>MAIELWTTRNDTTSVQAFYAAEAGLQKYKAALFQQYVWREQRGGTGGGGGCFTSLARGLDLDRDGTITPFVNNRLVLAQNEVVTDANGNPVGRYTATLYKDAQDDQLFTLVSEGTSGGAKARVQATFRISNSDYLEQAIFAGAGQANKWLNGGATIRGGVYVVGNPNDPDQYVIEANGNFALYNRYDLTTYSEVTNRVEPSYRQVQDLCASLRVQYGKISVGGSTQIGEPNNKVKGVFVGRGAQDITGENVGVCRNNKGVCTEAMGGFDLSDPPPFPTLDAKLDSDACSAYPTWRACLQGKAALRIQRIGNILSVASPPNATLSPSCLQAMQSGTLTLDTQSVDCTFTRLDGSRGGFRYTYTGGQELLEVFGDVVLEGIDAVLNRPVDYRAQSGSAKSATLAVLKLGGNGGNLDINGNLLPDATFGLFPNHALGFVAEGDIYQRGQHVMAPVYAGGTFRVVKGNVLFGSVISNQFCTTSAGNQMSCNASQKAEVVYIRIPKENRPALLPSLRGGKPVFQVLSYERRLEHHHHHH[3x]

Natural competence is the term used to describe the uptake of “naked” extracellular DNA by bacteria; it plays a significant role in horizontal genetic exchange. Previous work on T. thermophilus HB27 by Friedrich et al. identified a locus containing five open reading frames (ORFs) associated with natural competence. Four ORFs (pilA1 to pilA4 [pilA1-4]) were type IVa pilin-like genes, and a fifth, comZ, encoded an unusual and much larger protein that lacked some of the sequence features characteristic of pilin genes. Mutation of pilA1-3 and comZ leads to a loss of natural competence, although piliation is maintained.

ComZ was crystallized and the structure was determined to 2.72-Å resolution. The structure had three ComZ molecules in the asymmetric unit, but analysis by the protein interface analysis server PISA did not indicate any significant crystal contacts. ComZ was not identified as a type IV pilin by PilFind, presumably because it does not contain key characteristic sequence motifs; however, the N-terminal domain adopts a type IV pilin-like fold, suggesting that it forms a structural component of a pilus fiber. The second domain forms a complex β-solenoid structure, which is inserted between the penultimate and last β-strands in the pilin fold through two short linkers. From a comparison of the three chains, the relative orientation of the two domains is invariant. The closest match was the type II secretion system pseudopilin GspK, which forms the tip of a pseudopilus heterotrimeric complex (GspK/GspI/GspJ). In fact, the β-solenoid domain is placed in line with the central axis of the fiber, placing it in an ideal orientation to act as a tip adhesin. Protection against reductive dimethylation was used in combination with mass spectrometry and site-directed mutagenesis to identify two lysine residues in ComZ which are involved in DNA binding. They are located between the two domains in ComZ, on the opposite side from the predicted PilA2 binding site.>KFNDTLFGEMLHGYNNRTQHVNQGQVFQMTFRENNFIKDFPQLADGLLVIPLPVEEQCRGVLSEPLPDLQLLTGDIRYDEAMGYPMVQQWRVRSNLYRVKLSTITLAAGFTNVLKILTKESSREELLSFIQHYGSHYIAEALYGSELTCIIHFPSKKVQQQLWLQYQKETTELGSKKELKSMPFITYLSGLLTAQMLSDDQLISGVEIRCEEKGRCPSTCHLCRRPGKEQLSPTPVLLEINRVVPLYTLIQDNGTKEAFKSALMSSYWCSGKGDVIDDWCRCDLSAFDANGLPNCSPLLQPVLRLSPTVEPSSTVVSLEWVDVQPAIGTKVSDYILQHKKVDEYTDTDLYTGEFLSFADDLLSGLGT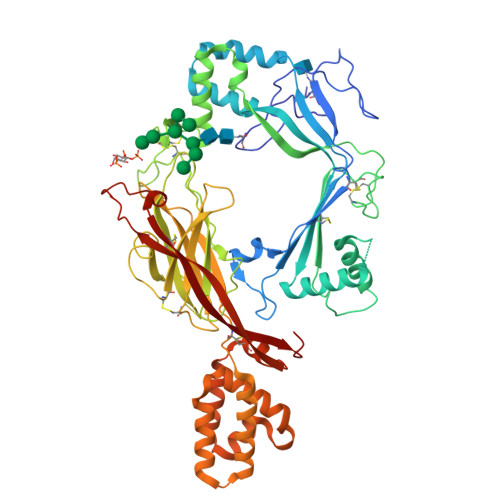SCVAAGRSHGEVPEVSIYSVIFKCLEPDGLYKFTLYAVDTRGRHSELSTVTLRTACPLVDDNKAEEIADKIYNLYNGYTSGKEQQMAYNTLMEVSASMLFRVQHHYNSHYEKFGDFVWRSEDELGPRKAHLILRRLERVSSHCSSLLRSAYIQSRVETVPYLFCRSEEVRPAGMVWYSILKDTKITCEEKMVSMARNTYGESKGR[4x]>[3x]MASQLDSGTPAREASSALRDGYRQAGVSGRVRSYLDLLAGLSDFREHFDGSDGFSLDLVDMADGPGEVTVICCAGTAAISGPHEFTRLAGALRGIAPVRAVPQPGYEEGEPLPSSMAAVAAVQADAVIRTQGDKPFVVAGHSAGALMAYALATELLDRGHPPRG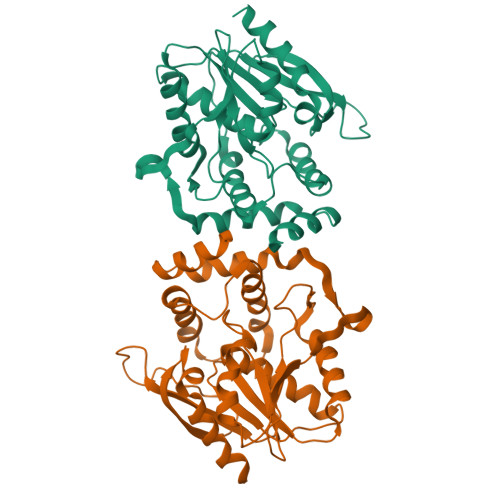VVLIDVYPPGHQDAMNAWLEELTATLFDRETVRMDDTRLTALGAYDRLTGQWRPRETGLPTLLVSAGEPMGPWPDDSWKPTWPFEHDTVAVPGDHFTMVQEHADAIARHIDAWLGGGNSSSVDKLAAALEHHHHHH>MNHKPKGTFKDYVRDRADLNKDKPVIPAAALAGYTGSGPIQLWQFLLELLTDKSCQSFISWTGDGWEFKLSDPDEVARRWGKRKNKPKMNYEKLSRGLRYYY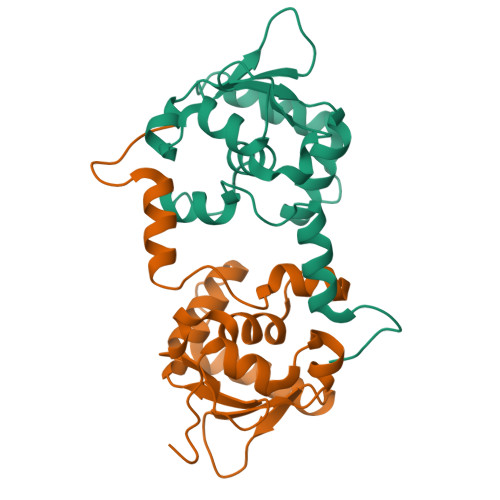DKNIIHKTAGKRYVYRFVCDLQSLLGYTPEELHAMLDVKPDADE[2x]3-[(3S,4R)-3-methyl-7-(7H-pyrrolo[2,3-d]pyrimidin-4-yl)-1,7-diazaspiro[3.4]octan-1-yl]-3-oxidanylidene-propanenitrile 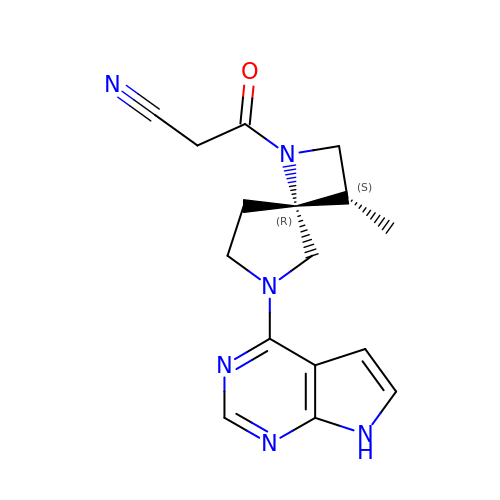| C16 H18 N6 O | LOWWYYZBZNSPDT-ZBEGNZNMSA-N> QGGAAAPISSHARLDKSNFQQPYITNRTFMLAKEASLADNNTDVRLIGEKLFHGVSMSERCYLMKQVLNFTLEEVLFPQSDRFQPYMQEVVPFLARLSNRLSTCHIEGDDLHIQRNVQKLKDTVKKLGESGEIKAIGELDLLFMSLRNACI;> PEDPSDLLQHVKFQSSNFENILTWDSGPEGTPDTVYSIEYKTYGERDWVAKKGCQRITRKSCNLTVETGNLTELYYARVTAVSAGGRSATKMTDRFSSLQHTTLKPPDVTCISKVRSIQMIVHP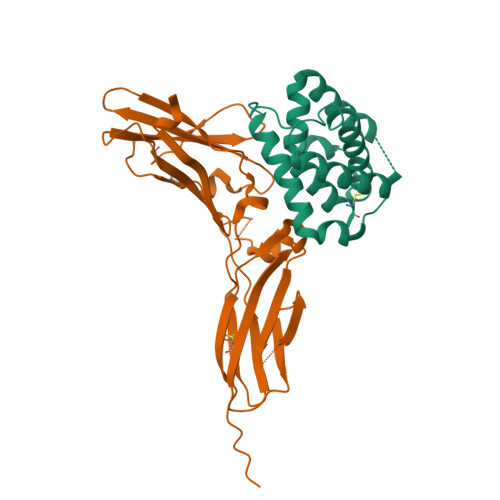TPTPIRAGDGHRLTLEDIFHDLFYHLELQVNRTYQMHLGGKQREYEFFGLTPDTEFLGTIMILVPTWAKESAPYMCRVKTLPDRTWT>[4x]MHAALTPLTNKYRFIDVQPLTGVLGAEITGVDLREPLDDSTWNEILDAFHTYQVIYFPGQAITNEQHIAFSRRFGPVDPVPILKSIEGYPEVQMIRREANESSRYIGDDWHADSTFLDAPPAAVVMRAIEVPEYGGDTGFLSMYSAWETLSPTMQATIEGLNVVHSATKVFGSLYQATNWRFSNTSVKVMDVDAGDRETVHPLVVTHPVTGRRALYCNQVYCQKIQGMTDAESKSLLQFLYEHA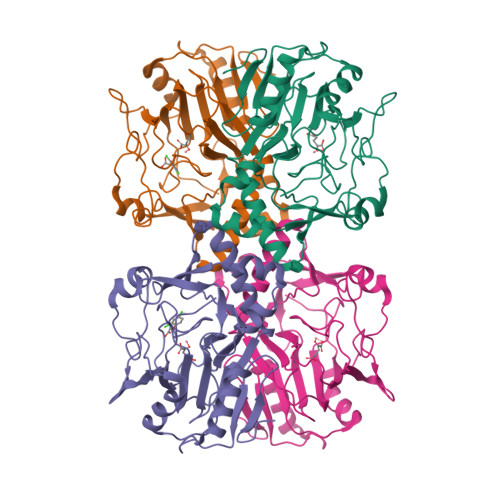TQFDFTCRVRWKKDQVLVWDNLCTMHRAVPDYAGKFRYLTRTTVAGDKPSR>[2x]MISKEYHIDEEVGFALPNPQENLPDFYNDWMFIAKHLPDLIESGQLRERVEKLNMLSIDHLTDHKSQRLARLVLGCITMAYVWGKGHGDVRKVLPR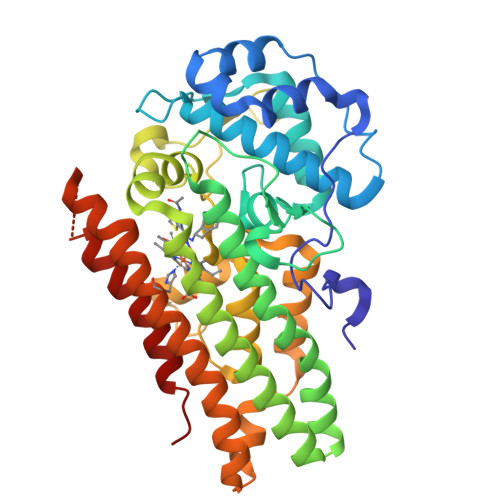NIAVPYCQLSKKLELPPILVYADCVLANWKKKDPNKPLTYENMDVLFSFRDGDCSKGFFLVSLLVEIAAASAIKVIPTVFKAMQMQERDTLLKALLEIASCLEKALQVFHQIHDHVNPKAFFSVLRIYLSGWKGNPQLSDGLVYEGFWEDPKEFAGGSAGQSSVFQCFDVLLGIQQTAGGGHAAQFLQDMRRYMPPAHRNFLCSLESNPSVREFVLSKGDAGLREAYDACVKALVSLRSYHLQIVTKYILIPASQQPKENKTSEDPSKLEAKGTGGTDLMNFLKTVRSTTEKSLLKE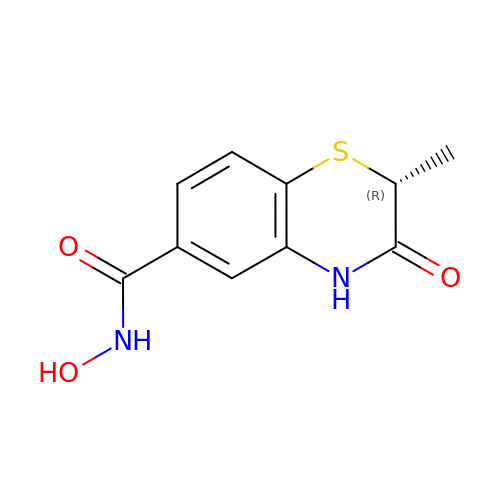(2R)-2-methyl-3-oxo-4H-1,4-benzothiazine-6-carbohydroxamic acid | C10 H10 N2 O3 S | YALBEYHVOFQECJ-RXMQYKEDSA-N>[2x]MVIPAGKLERVDPTTVRQEGPWADPAQAVVQTGPNQYTVYVLAHQWYYQPNPIEVPQGAEIVFKITSADVLHGFHVEGTNINVEVLPGEVSTVRYTFKRPGEYRIICSEICGTNHAFMFG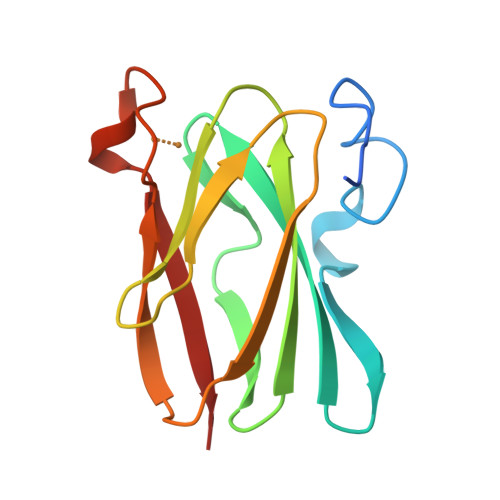TIVVKE>LPNAEDVDMPWDSDVFAVPSGYNAPQQVHITQGDYEGRGVIISWTTPYDKAGANKVFYWSENSKSQKRAMGTVVTYKYYNYTSAFIHHCTIKDLEYDTKYYYRLGFGDAKRQFWFVTPPKPGPDVPYVFGLIGDIGQTHDSNTTLTHYEQNSAKGQAVLFMGDLSYSNRWPNHDNNRWDTWGRFSERSVAYQPWIWTAGNHEIDYAPDIGEYQPFVPFTNRYPTPHEASGSGDPLWYAIKRASAHIIVLSSYSGFVKYSPQYKWFTSELEKVNRSETPWLIVLVHAPLYNSYEAHYMEGEAMRAIFEPYFVYYKVDIVFSGHVHSYERSERVSNVAYNIVNAKCTPVSDESAPVYITI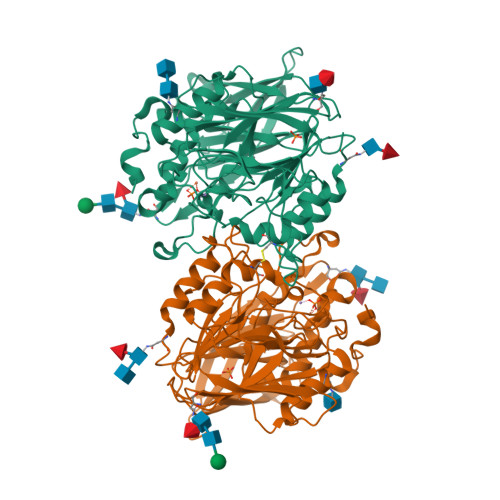GDGGNSEGLASEMTQPQPSYSAFREASFGHGIFDIKNRTHAHFSWHRNQDGASVEADSLWLLNRYWAS[2x]> MAHHHHHHMASKQHAHILSLARSMIPPLHPKLHKGQAGRIGVLGGSGDYSGAPYFSSMGAMRFGADLAHVICEPSAGAVIKTYSPDLIV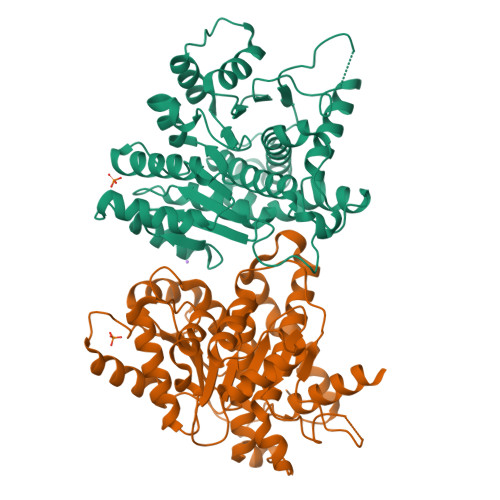HTILDPQKSREDIRSALKGVMSRLHVLIIGPGLGRDDHMQSCAKIAFELAKDMEQMGVVVDADGLWLVQNEPKVVMDWPGVPRIILTPNVMEFKRLCDTMKINASGPHTSLCPQLATALGNATIIQKGPSDIISNGLKIPFALLSDESEEEQNYLEVKVEGGLKRVGGQGDILSGSTGVLLAWGSEWVRGTYEHVGHPPPQDKAIKENIPVLAAYGASTFNRTVSKRGFQKKGRSMVTGDLVDMVGEVYEEVFGNPGEVEGRGKL pmcPeptide arginases are a recently discovered enzyme family (pfam12640) catalyzing the hydrolysis of arginine residues incorporated in a peptide chain to ornithine (Orn) units, constituting an unprecedented post-translational modification. The first characterized peptide arginase representative is OspR (OSCI_RS22075) from the cyanobacterium Kamptonema sp. (formerly Oscillatoria) PCC 6506. OspR hydrolyzes two arginine residues to ornithines in the precursor peptide OspA during the biosynthesis of landornamide A, a member of the proteusin family of RiPPs with antiviral activity toward lymphocytic choriomeningitis virus. Peptide arginases are weakly similar to the well-characterized family of conventional arginases (EC 3.5.3.1, also known as l-arginine amidinohydrolases) that hydrolyze free l-arginine monomers to l-ornithine and urea.

Here, we report the first crystal structure of a peptide arginase at a resolution of 2.6 Å. The structure of OspR reveals a three-layered α-β-α sandwich arrangement, which is a fold shared by all arginases.30 Apart from this similarity, the macromolecular assembly of OspR shows major differences compared to other arginases. As confirmed by analytical size exclusion chromatography, OspR forms a homodimer in solution. The dimer contact region is almost exclusively established by an additional domain (residues Ser170-Ser234), which is absent in conventional arginases. The narrow region occurring in the center of the OspR homodimer forms a large surface-exposed cleft, which presumably acts as the binding site for the 10 kDa leader region of OspA. The base of the negatively charged cavity accommodates a binuclear manganese cluster typical for arginases. MnA of OspR is coordinated by His12 and Asp43, whereas MnB binds to His41 and Asp167. Asp39 and Asp165 complex both metal ions. Interestingly, the OspR structure features an acetate molecule that is bound at the substrate binding site serving as a mimic for the guanidine moiety of the actual substrate. Furthermore, the established arginase mechanism features a histidine residue that serves as an important proton shuttle. This histidine is replaced by Ile73 in OspR, a residue which is unable to perform the same task.

>GSAKIPFYIMEEHNEAFFIWHYAVAEGWINKNQNTLLHVDEHSDLVVPILNSSLKSVNENIKRVHDFTYSELTIANFIYPALYQGVFSQVYWLRQKHDPKLNGQKQLNIYSHQGEGKRLILKSKVDFNNLFNPDCKSFTITPLNAQDDLSSEESKKLNKSVILDIDIDYFSCDNVSGEYLEVEITEEAYYDYINNLYNKLRICWGGNASVKYMDGKYYFCIIQPDKLVAENLKVSEDAIVERIDALIDFLKVNEIQPKLIDVCRSRLSGYTPNDQWEFIENTLVEKLSSIYEFEPIFVSELSKKVLVEV[4x]>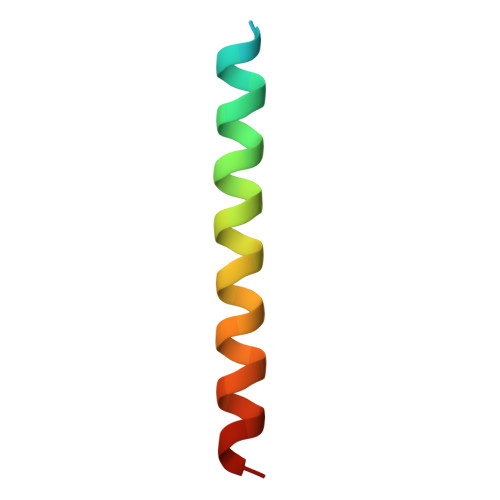 XVALDPXDISIVLNKIKSQLEESKEWIRRSNKILDSIX> MPDAESRSQVTAKAAPPPAPKTNSIEQVRYICSIGAMHSASAIPRVIPITHCGPGCADKQFMNVAFYNGFQGGGYGGGAVVPSTNATEREVVFGGAERLDELIGASLQVLDADLFVVLTGCIPDLVGDDIGSVVGPYQKRGVPIVYAETGGFRGNNFTGHELVTKAIIDQFVGDYDAERDGAREPHTVNVWSLLPYHNTFWRGDLTEIKRLLEGIGLKVNILFGPQSAGVAEWKAIPRAGFNLVLSPWLGLDTARHLDRKYGQPTLHRPIIPIGAKETGAFLREVAAFAGLDSAVVEAFITAEEAVYYRYLEDFTDFYAEYWWGLPAKFAVIGDSAYNLAL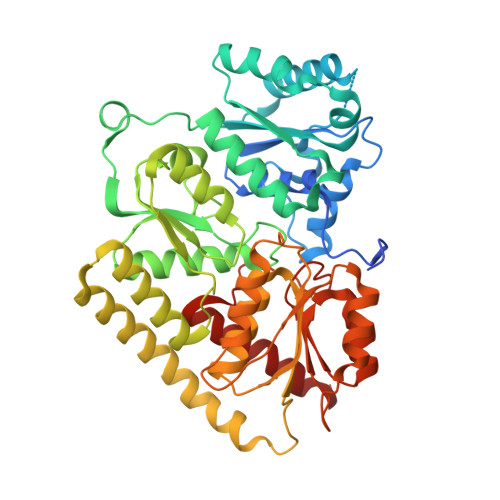TKFLVNQLGLIPGLQIITDNPPEEVREDIRAHYHAIADDVATDVSFEEDSYTIHQKIRATDFGHKAPILFGTTWERDLAKELKGAIVEVGFPASYEVVLSRSYLGYRGALTLLEKIYTTTVSASA> GSFLP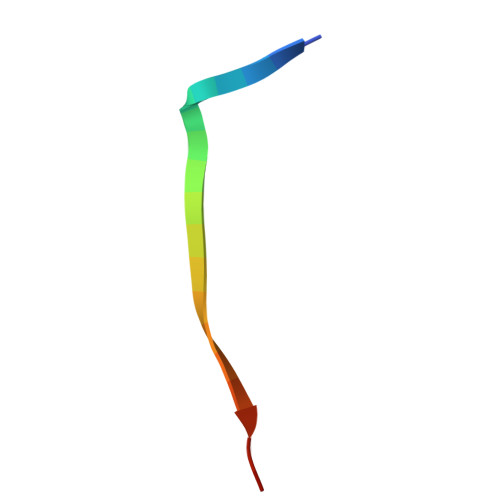NSEQQKSVDIVASSP>[2x]MASGSCQGCEEDEETLKKLIVRLNNVQEGKQIETLVQILEDLLVFTYSEHASKLFQGKNIHVPLLIVLDSYMRVASVQQVGWSLLCKLIEVCPGTMQSLMGPQDVGNDWEVLGVHQLILKMLTVHNASVNLSVIGLKTLDLLLTSGKITLLILDEESDIFMLIFDAMHSFPANDEVQKLGCKALHVLFERVSEEQLTEFVENKDYMILLSALTNFKDEEEIVLHVLHCLHSLAIPCNNVEVLMSGNVRCYNIVVEAMKAFPMSERIQEVSCCLLHRLTLGNFFNILVLNEVHEFVVKAVQQYPENAALQISALSCLALLTETIFLNQDLEEKNENQENDDEGEEDKLFWLEACYKALTWHRKNKHVQEAACWALNNLLMYQNSLHEKIGDEDGHFPAHREVMLSMLMHSSSKEVFQASANALSTLLEQNVNFRKILLSKGIHLNVLELMQKHIHSPEVAESGCKMLNHLFEGSNTSLDIMAAVVPKILTVMKRHETSLPVQLEALRAILHFIVPGMPEESREDTEFHHKLNMVKKQCFKNDIHKLVLAALNRFIGNPGIQKCGLKVISSIVHFPDALEMLSLEGAMDSVLHTLQMYPDDQEIQCLGLSLIGYLITKKNVFIGTGHLLAKILVSSLYRFKDVAEIQTKGFQTILAILKLSASFSKLLVHHSFDLVIFHQMSSNIMEQKDQQFLNLCCKCFAKVAMDDYLKNVMLERACDQNNSIMVECLLLLGADANQAKEGSSLICQVCEKESSPKLVELLLNSGSREQDVRKALTISIGKGDSQIISLLLRRLALDVANNSICLGGFCIGKVEPSWLGPLF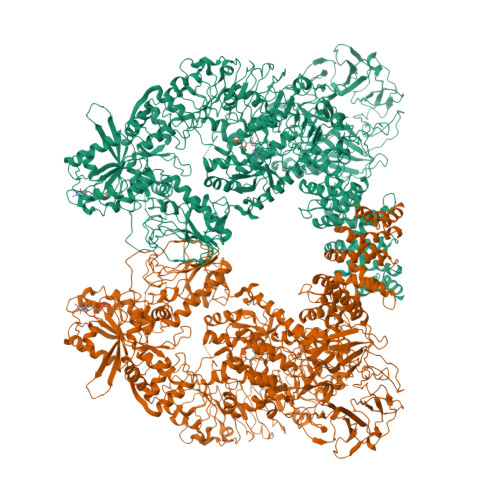PDKTSNLRKQTNIASTLARMVIRYQMKSAVEEGTASGSDGNFSEDVLSKFDEWTFIPDSSMDSVFAQSDDLDSEGSEGSFLVKKKSNSISVGEFYRDAVLQRCSPNLQRHSNSLGPIFDHEDLLKRKRKILSSDDSLRSSKLQSHMRHSDSISSLASEREYITSLDLSANELRDIDALSQKCCISVHLEHLEKLELHQNALTSFPQQLCETLKSLTHLDLHSNKFTSFPSYLLKMSCIANLDVSRNDIGPSVVLDPTVKCPTLKQFNLSYNQLSFVPENLTDVVEKLEQLILEGNKISGICSPLRLKELKILNLSKNHISSLSENFLEACPKVESFSARMNFLAAMPFLPPSMTILKLSQNKFSCIPEAILNLPHLRSLDMSSNDIQYLPGPAHWKSLNLRELLFSHNQISILDLSEKAYLWSRVEKLHLSHNKLKEIPPEIGCLENLTSLDVSYNLELRSFPNEMGKLSKIWDLPLDELHLNFDFKHIGCKAKDIIRFLQQRLKKAVPYNRMKLMIVGNTGSGKTTLLQQLMKTKKSDLGMQSATVGIDVKDWPIQIRDKRKRDLVLNVWDFAGREEFYSTHPHFMTQRALYLAVYDLSKGQAEVDAMKPWLFNIKARASSSPVILVGTHLDVSDEKQRKACMSKITKELLNKRGFPAIRDYHFVNATEESDALAKLRKTIINESLNFKIRDQLVVGQLIPDCYVELEKIILSERKNVPIEFPVIDRKRLLQLVRENQLQLDENELPHAVHFLNESGVLLHFQDPALQLSDLYFVEPKWLCKIMAQILTVKVEGCPKHPKGIISRRDVEKFLSKKRKFPKNYMTQYFKLLEKFQIALPIGEEYLLVPSSLSDHRPVIELPHCENSEIIIRLYEMPYFPMGFWSRLINRLLEISPYMLSGRERALRPNRMYWRQGIYLNWSPEAYCLVGSEVLDNHPESFLKITVPSCRKGCILLGQVVDHIDSLMEEWFPGLLEIDICGEGETLLKKWALYSFNDGEEHQKILLDDLMKKAEEGDLLVNPDQPRLTIPISQIAPDLILADLPRNIMLNNDELEFEQAPEFLLGDGSFGSVYRAAYEGEEVAVKIFNKHTSLRLLRQELVVLCHLHHPSLISLLAAGIRPRMLVMELASKGSLDRLLQQDKASLTRTLQHRIALHVADGLRYLHSAMIIYRDLKPHNVLLFTLYPNAAIIAKIADYGIAQYCCRMGIKTSEGTPGFRAPEVARGNVIYNQQADVYSFGLLLYDILTTGGRIVEGLKFPNEFDELEIQGKLPDPVKEYGCAPWPMVEKLIKQCLKENPQERPTSAQVFDILNSAELVCLTRRILLPKNVIVECMVATHHNSRNASIWLGCGHTDRGQLSFLDLNTEGYTSEEVADSRILCLALVHLPVEKESWIVSGTQSGTLLVINTEDGKKRHTLEKMTDSVTCLYCNSFSKQSKQKNFLLVGTADGKLAIFEDKTVKLKGAAPLKILNIGNVSTPLMCLSESTNSTERNVMWGGCGTKIFSFSNDFTIQKLIETRTSQLFSYAAFSDSNIITVVVDTALYIAKQNSPVVEVWDKKTEKLCGLIDCVHFLREVTVKENKESKHKMSYSGRVKTLCLQKNTALWIGTGGGHILLLDLSTRRLIRVIYNFCNSVRVMMTAQLGSLKNVMLVLGYNRKNTEGTQKQKEIQSCLTVWDINLPHEVQNLEKHIEVRKELAEKMRRTSVE>MAMTVTEVDLPPIYCPLESAIHPRVHEVEKRAVEWIRRSGMCASEEERAWVIATHSADFFARFAPTAADEDRLLATSLFVYWLFAFDDHRCDNGPLSTRPAQFNALAGRVQRALEAPSAEDNGDRFVPALQDIARRFRSFGTPTQVRRFVHAHRAWLSGVAWQIGNQARGHMPGLDDYLAMRLLSAGGEPTFAMLEIATGAEVPDREMHRPAVRALTEMAIMVAALDNDRHSLRKELSRGHTDQ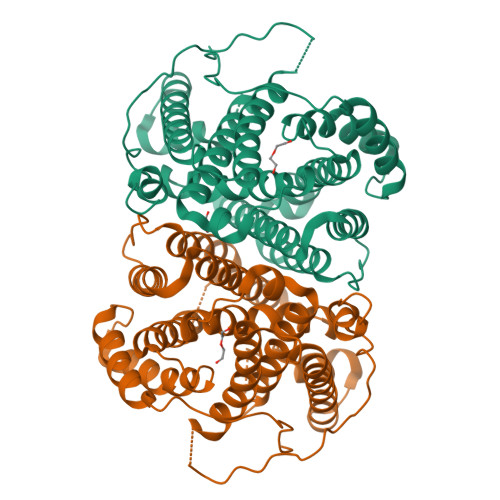NIYSVLMHHRGMSLQEAVEEATKLRDRILLRFLELHDRVRPGAGAELSTYLQGLRHGIRGNAEWGLRVPRYLSLGRVPDPMEDAPLTWAESPSDSSPSPLPGAPSIAWWWDDALLGA[2x]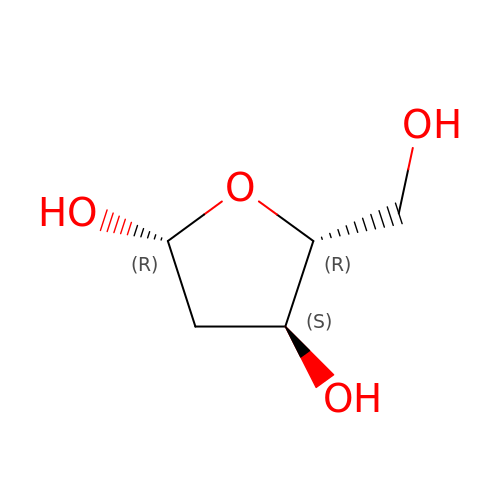2-deoxy-beta-D-erythro-pentofuranose | C5 H10 O4 | PDWIQYODPROSQH-VPENINKCSA-N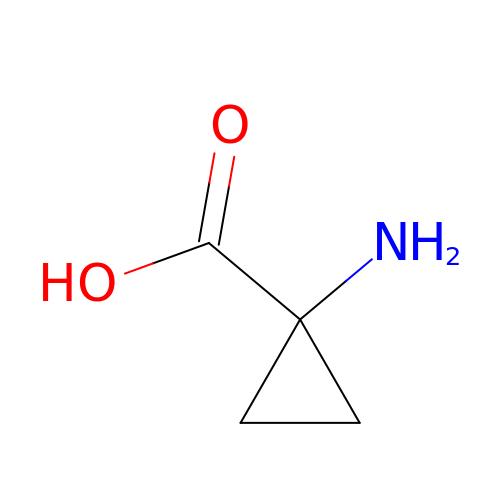1-AMINOCYCLOPROPANECARBOXYLIC ACID | C4 H7 N O2 | PAJPWUMXBYXFCZ-UHFFFAOYSA-N> MGSSHHHHHHSSGLVPRGSMGQEPRTLPPSPNWYCARCSDAVPGGLFGFAARTSVFLVRVGPGAGESPGTPPFRVIGELVGHTERVSGFTFSHHPGQYNLCATSSDDGTVKIWDVETKTVVTEHALHQHTISTLHWSPRVKDLIVSGDEKGVVFCYWFNRNDSQHLFIEPRTIFCLTCSPHHEDLVAIGYKDGIVVIIDISKKGEVIHRLRGHDDEIHSIAWCPLPGEDCLSINQEETSEEAEITNGNAVAQAPVTKGCYLATGSKDQTIRIWSCSRGRGVMILKLPFLKRRGGGIDPTVKERLWLTLHWPSNQPTQLVSSCFGGELLQWDLTQSWRRKYTLFSASSEGQNHSRIVFNLCPLQTEDDKQLLLSTSMDRDVKCWDIATLECSWTLPSLGGFAYSLAFSSVDIGSLAIGVGDGMIRVWNTLSIKNNYDVKNFWQGVKSKVTALCWHPTKEGCLAFGTDDGKVGLYDTYSNKPPQISSTYHKKTVYTLAWGPPVPPMSLGGEGDRPSLALYSCGGEGIVLQHNPWKLSGEAFDINKLIRDTNS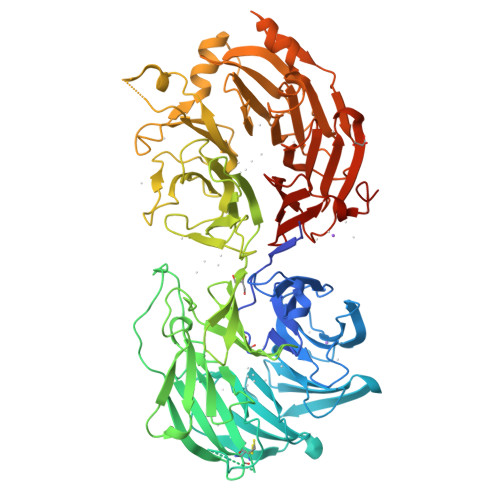IKYKLPVHTEISWKADGKIMALGNEDGSIEIFQIPNLKLICTIQQHHKLVNTISWHHEHGSQPELSYLMASGSNNAVIYVHNLKTVIESSPESPVTITEPYRTLSGHTAKITSVAWSPHHDGRLVSASYDGTAQVWDALREEPLCNFRGHQGRLLCVAWSPLDPDCIYSGADDFCVHKWLTSMQDHSRPPQGKKSIELEKKRLSQPKA>[2x]MPSLFDPIRFGAFTAKNRIWMAPLTRGRATRDHVPTEIMAEYYAQRASAGLIISEATGISQEGLGWPYAPGIWSDAQVEAWLPITQAVHDAGGLIFAQLWHMGRMVPSNVSGMQPVAPSASQ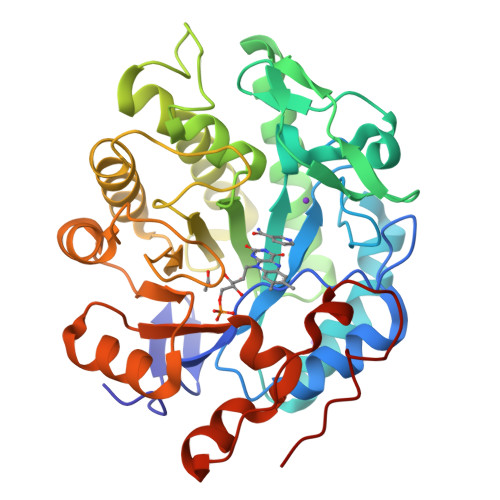APGLGHTYDGKKPYDVARALRLDEIPRLLDDYEKAARHALKAGFDGVQIHAANGYLIDEFIRDSTNHRHDEYGGAVENRIRLLKDVTERVIATIGKERTAVRLSPNGEIQGTVDSHPEQVFIPAAKMLSDLDIAFLGMREGAVDGTFGKTDQPKLSPEIRKVFKPPLVLNQDYTFETAQAALDSGVADAISFGRPFIGNPDLPRRFFEKAPLTKDVIETWYTQTPKGYTDYPLLGD5-cyclohexyl-3-(pyridin-4-yl)-1,2,4-oxadiazole 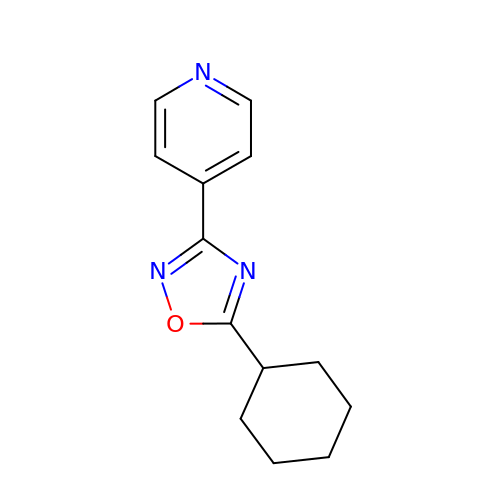| C13 H15 N3 O | XXTHMVRJMJIERU-UHFFFAOYSA-N> CVHHIKRRDIVLKWELGEGAFGKVFLAECHNLLPEQDKMLVAVKALKEASESARQDFQREAELLTMLQHQHIVRFFGVCTEGRPLLMVFEYMRHGDLNRFLRSHGPDAKLLAGGEDVAPGPLGLGQLLAVASQVAAGMVYLAGLHFVHRDLATRNCLVGQGLVVKIGDFGMSRDIYSTDYYRVGGRTMLPIRWMPPESILYRKFTTESDVWSFGVVLWEIFTYGKQPWYQLSNTEAIDCI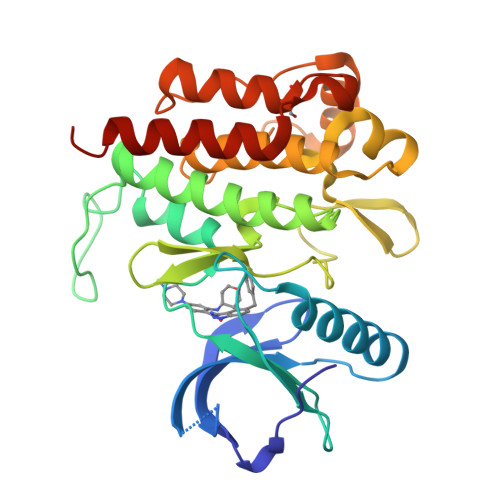TQGRELERPRACPPEVYAIMRGCWQREPQQRHSIKDVHARLQALAQAHHHHHH>MQSEQWRSLSNVVWGKDLPAFTYAFSKTPLVLYDGGTTKQVGTYNFPVSKGMAGVYMSLEPGAIRELHWHANAAEWAYVMEGRTRITLTSPEGKVEIADVDKGGLWYFPRGWGHSIEGIGPDTAKFLLVFNDGTFSEGATFSVTDWLSHTPIAWVEENLGWTAAQVAQLPKKQVYISSYGPASGPLASATPQGQTAKIEVPHTHNLLGQQPLVSLGGNELRLASAKEFPGSFNMTGALIHLEPGAMRQLHWHPNADEWQYVLDGEMDLTVFASEGKASVSRLQQGDVGYVPKGYGHAIRNSSQKPLDIVVVFNDGDYQSIDLSTWLASNPSSVLGNTFQISPELTKKLPVQDTIFSLPTQP[3x]

Here we use a cyanobacterial MnII-cupin (MncA) as a metal trap, to test predictions of metalation. Two metal-binding cupins, MnII-MncA and CuII-CucA, were discovered in the periplasm of a cyanobacterium (Synechocystis PCC 6803), notably binding metals from different ends of the Irving-Williams series yet exploiting similar folds and identical metal-binding residues. While the copper-cupin is secreted unfolded via the Sec-system, the MnII-cupin is a Tat-substrate which folds and kinetically traps the less competitive metal in the cytosol before secretion. MncA is an MnII-dependent oxalate decarboxylase (inactive with copper or ZnII), and the related cytosolic OxdC from Bacillus subtilis trapped either MnII or CoII in E. coli depending on media metal supplementation.

However, MncA might adopt non-native folds with non-cognate metals. Abnormally coordinated metals might not be kinetically trapped. NiII often prefers four-coordinate, planar geometries, and NiII-MncA was chosen for structural analysis. A crystal structure of NiII-MncA (1.6 Å resolution), shows the bi-cupin fold of MnII-MncA with a metal atom in each cupin domain. Each MnII atom is coordinated to three histidine and one glutamate residue with non-protein ligands completing hexacoordinate MnII coordination spheres. NiII-MncA has similar coordination environments with no channel to the amino-terminal NiII and a narrow channel to the carboxy-terminal site analogous to MnII-MncA. The channel is presumed to allow substrate access to catalytic MnII. The substrate site was gratuitously occupied by acetate in the MnII structure and with glycine in the crystalised NiII-form. The narrow hydrophobic channel is unlikely to allow NiII exchange and thus both NiII atoms appear trapped.Rab GTPases act as molecular switches and cycle between a GDP “off” state and a GTP-bound “on” state. The Rab11 proteins are master regulators of the surface expression of receptors. The mammalian ortholog of REI-1, SH3-binding protein 5 (SH3BP5), also has GEF activity toward Rab11 and was shown to be selective for Rab11 over Rab526. Detailed biochemical studies reveal that SH3BP5 is highly selective for Rab11 isoforms, with no activity toward any of the most evolutionarily similar Rab GTPases.

To understand the molecular basis of how SH3BP5 mediates Rab11A nucleotide exchange, we determined the structure of the N-terminal GEF domain of SH3BP5 bound to full-length Q70L Rab11A to a final resolution of 3.1 Å. The Q70L construct of Rab11 was used for structural studies as the marginally increased GEF rate for Q70L vs. WT suggested Q70L might form a slightly more stable complex with SH3BP5. The structure is composed of four complexes of SH3BP5-Rab11A per asymmetric unit, with each of the copies in the asymmetric unit sharing an overall similar architecture. The GEF domain of SH3BP5 is composed of a coiled coil that is kinked to form an overall v-shape. The v is composed of four long α-helices (α1–α4), with a small helix connecting helices α2 α3. Nucleotide-free Rab11A was bound to the GEF domain of SH3BP5 at one end of the v at a surface composed of the N terminus of helix α1 and the C terminus of helix α4 of the coiled coil. The SH3BP5-Rab11 interface is composed of a large extended, primarily hydrophobic interface (~1250 Å2). Comparison of the structure of nucleotide-free Rab11A bound to SH3BP5 compared with Rab11A bound to either GDP or GTP reveals an extensive rearrangement of switch I41, with only limited conformational changes in switch II. The main difference is in the conformation of F36 and I44 in Rab11. These residues pack directly against each other, which requires a constrained conformation of switch I. This constrained orientation of the highly conserved F36 and I44 residues is unique compared with previously solved Rab-GEF structures.

>GSHMGTRDDEYDYLFKVVLIGDSGVGKSNLLSRFTRNEFNLESKSTIGVEFATRSIQVDGKTIKAQIWDTAGLERYRAITSAYYRGAVGALLVYDIAKHLTYENVERWLKELRDHADSNIVIMLVGNKSDLRHLRAVPTDEARAFAEKNGLSFIETSALDSTNVEAAFQTILTEIYRIVSQKQMSDRRENDMSPSNNVVPIHVPPTTENKPKVQCCQNI[4x];>[4x]GMDAALKRSRSEEPAEILPPARDEEEEEEEGMEQGLEEEEEVDPRIQGELEKLNQSTDDINRRETELEDARQKFRSVLVEATVKLDELVKKIGKAVEDSKPYWEARRVARQAQLEAQKATQDFQRATEVLRAAKETISLAEQRLLEDDKRQFDSAWQEMLNHATQRVMEAEQTKTRSELVHKETAARYNAAMGRMRQLEKKLKRAINKSKPYFELKAKYYVQLEQLKKTVDDLQAKLTLAKGEYKMALKNLEMISDEIHERRRSSA>KHTLPDLPFDYADLEPVISHEIMQLHHQKHHATYVNNLNQIEEKLHEAVSKGNLKEAIALQPALKFNGGGHINHSIFWTNL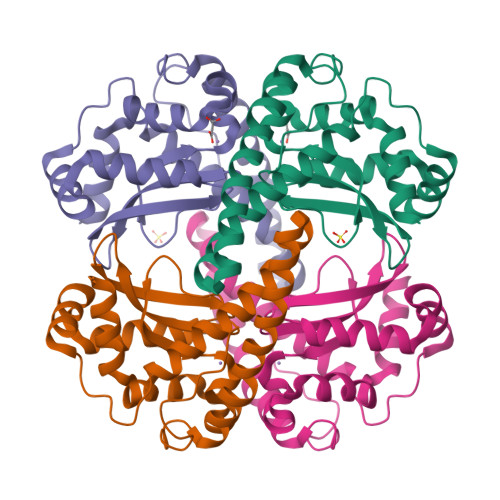AKDGGEPSKELMDTIKRDFGSLDNLQKRLSDITIAVQGSGWGWLGYCKKDKILKIATCANQDPLEGMVPLFGIDVWEHAYYLQYKNVRPDYVHAIWKIANWKNISERFANARQ[2x]The human BEST1 gene encodes a protein (BESTROPHIN1, or BEST1) that is predominantly expressed in retinal pigment epithelium (RPE). BEST1 localizes to the basolateral membrane of RPE, and has been functionally identified as a CaCC in heterologous expression studies. The simplest and most logical conclusion based on our results is that BEST1 functions as the surface CaCC to generate Ca2+-dependent Cl- current in human RPE. Since the structure of BEST1 has not been solved, we generated a three-dimensional human homology model based on our previously solved Klebsiella pneumoniae bestrophin (KpBest) structure and a chicken bestrophin1 (cBest1) structure.

On the other hand, I201 resides in a loop between S2h and S3a, surrounded by hydrophobic residues V114, A195, L207, and L210, which are conserved among species and thus probably important for the channel function. As the Ile to Thr substitution changes a hydrophobic residue to a polar residue, which weakens the hydrophobic interactions, this mutation may change the channel property by altering the local interplays between spatially adjacent subunits, but will unlikely disrupt the channel structure as its localization on a loop renders flexibility. Sequence alignment reveals that BEST1 P274 is identical while I201 has a highly conservative substitution in KpBest (P239 and L177, respectively), prompting us to test the predictions from the BEST1 homology model with the corresponding KpBest mutants (P239R and L177T, respectively) expressed from E. coli. Purified KpBest mutant proteins were set for crystal growing. While no crystal was grown with KpBest P239R, well-diffracted KpBest L177T crystals were obtained under the same condition as KpBest WT, and the structure was solved to 3.1 Å resolution (Figure 8—source data 1). The KpBest L177T structure mirrors that of KpBest WT, with all-atom alignment RMSD (root-mean-square deviation) in a protomer 0.4 Å (Coot LSQ superpose). However, superposition of KpBest WT with the L177T mutant based on the alignment of single chain residues 174–180 showed an obvious shift of the TM region. By contrast, no currents were obtained with KpBest P239R, while currents with reduced unitary conductance (mean amplitude 1.5 pA) were recorded with KpBest L177T, suggesting that the BEST1 P274R and I201T mutations result in a complete and partial loss of single channel activity, respectively. The structure of KpBest I177T suggests that the BEST1 I201T mutation does not alter the pentameric conformation of the channel. The condition contained 0.05 M zinc acetate, 6% v/v ethylene glycol, 0.1 M sodium cacodylate, pH 6.0, and 6.6 % w/v PEG 8000. Taken together, we concluded that P274R is a null mutation that abolishes both plasma membrane localization and channel activity of BEST1 due to structural disruption, whereas I201T is a partial loss-of-function mutation that retains plasma membrane localization and Ca2+ sensitivity of BEST1 caused by minor structural alterations.

>[5x]SNAMIIRPEQHWFLRLFDWHGSVLSKIIFRLLLNVLMSIIAIISYQWYEQLGIHLTVAPFSLLGIAIAIFLGFRNSASYSRFVEARNLWGTVLIAERTLVRQLRNILPAEHDAHRRIVSYLVAFSWSLKHQLRKTDPTADLRRLLPEERVTEILASSMPTNRILLLAGNEIGQLREAGKTSDITYGLMDNKLDELAHVLGGCERLATTPVPFAYTLILQRTVYLFCTLLPFALVGDLHYMTPFVSVFISYTFLSWDSLAEELEDPFGTAANDLPLNAMCNTIERNLLDMTGQHPLPE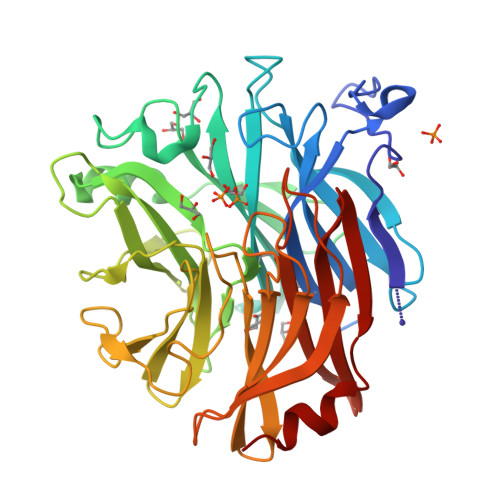> EKSVVFKAEGEHFTDQKGNTIVGSGSGGTTKYFRIPAMCTTSKGTIVVFADARHNTASDQSFIDTAAARSTDGGKTWNKKIAIYNDRVNSKLSRVMSPTCIVANIQGRETILVMVGKWNNNDKTWGAYRDKAPDTDWDLVLYKSTDDGVTFSKVETNIHDIVTKNGTISAMLGGVGSGLQLNDGKLVFPVQMVRTKNITTVLNTSFIYSTDGITWSLPSGYCEGFGSENNIIEFNASLVNNIRNSGLRRSFETKDFGKTWTEFPPMDKKVDNRNHGVQGSTITIPSGNKLVAAHSSAQNKNNDYTRSDISLYAHNLYSGEVKLIDDFYPKVGNASGAGYSCLSYRKNVDKETLYVVYEANGSIEFQDLSRHLPVIKSYN> MGSLVCVGTGLQLAGQISVLSRSYIEHADIVFSLLPDGFSQRWLTKLNPNVINLQQFFAQNGEVKNRRDTYEQMVNAILD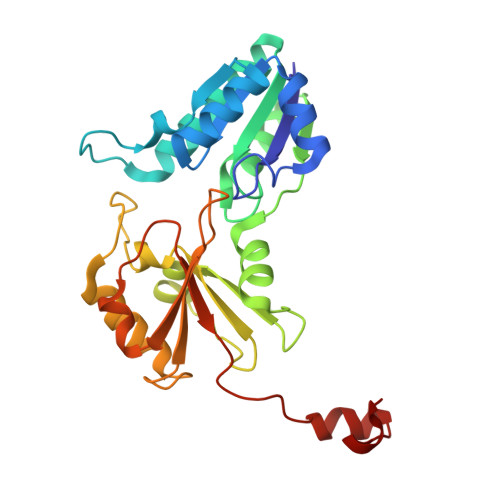AVRAGKKTVCALYGHPGVFACVSHMAITRAKAEGFSAKMEPGISAEACLWADLGIDPGNSGHQSFEASQFMFFNHVPDPTTHLLLWQIAIAGEHTLTQFHTSSDRLQILVEQLNQWYPLDHEVVIYEAANLPIQAPRIERLPLANLPQAHLMPISTLLIPPAKKLEYNYAILAKLGIGPEDLG> SNAMTQFEGFTNLYQVSKTLRFELIPQGKTLKHIQEQGFIEEDKARNDHYKELKPIIDRIYKTYADQCLQLVQLDWENLSAAIDSYRKEKTEETRNALIEEQATYRNAIHDYFIGRTDNLTDAINKRHAEIYKGLFKAELFNGKVLKQLGTVTTTEHENALLRSFDKFTTYFSGFYENRKNVFSAEDISTAIPHRIVQDNFPKFKENCHIFTRLITAVPSLREHFENVKKAIGIFVSTSIEEVFSFPFYNQLLTQTQIDLYNQLLGGISREAGTEKIKGLNEVLNLAIQKNDETAHIIASLPHRFIPLFKQILSDRNTLSFILEEFKSDEEVIQSFCKYKTLLRNENVLETAEALFNELNSIDLTHIFISHKKLETISSALCDHWDTLRNALYERRISELTGKITKSAKEKVQRSLKHEDINLQEIISAAGKELSEAFKQKTSEILSHAHAALDQPLPTTLKKQEEKEILKSQLDSLLGLYHLLDWFAVDESNEVDPEFSARLTGIKLEMEPSLSFYNKARNYATKKPYSVEKFKLNFQMPTLASGWDVNKEKCNGAILFVKNGLYYLGIMPKQKGRYKALSFEPTEKTSEGFDKMYYDYFPDAAKMIPKCSTQLKAVTAHFQTHTTPILLSNNFIEPLEITKEIYDLNNPEKEPKKFQTAYAKKTGDQKGYREALCKWIDFTRDFLSKYTKTTSIDLSSLRPSSQYKDLGEYYAELNPLLYHISFQRIAEKEIMDAVETGKLYLFQIYNKDFAKGHHGKPNLHTLYWTGLFSPENLAKTSIKLNGQAELFYRPKSRMKRMAHRLGEKMLNKKLKDQKTPIPDTLYQELYDYVNHRLSHDLSDEARALLPNVITKEVSHEIIKDRRFTSDKFFFHVPITLNYQAANSPSKFNQRVNAYLKEHPETPIIGIDRGERNLIYITVIDSTGKILEQRSLNTIQQFDYQKKLDNREKERVAARQAWSVVGTIKDLKQGYLSQVIHEIVDLMIHYQAVVVLENLNFGFKSKRTGIAEKAVYQQFEKMLIDKLNCLVLKDYPAEKVGGVLNPYQLTDQFTSFAKMGTQSGFLFYVPAPYTSKIDPLTGFVDPFVWKTIKNHESRKHFLEGFDFLHYDVKTGDFILHFKMNRNLSFQRGLPGFMPAWDIVFEKNETQFDAKGTPFIAGKRIVPVIENHRFTGRYRDLYPANELIALLEEKGIVFRDGSNILPKLLENDDSHAIDTMVALIRSVLQMRNSNAATGEDYINSPVRDLNGVCFDSRFQNPEWPMDADANGAYHIALKGQLLLNHLKESKDLKLQNGISNQDWLAYIQELRN

CRISPR-Cas12a uses guide RNAs to identify complementary ∼20-nucleotide sequences in genomic DNA to facilitate binding and double-strand cleavage. To engage DNA, Cas12a probes nucleotides immediately adjacent to 5′-TTTV-3′ protospacer adjacent motifs (PAMs) to test for guide RNA hybridization (1–3). We used cryo-electron microscopy (cryo-EM) to determine structures of a complex between Acidaminococcus sp. Cas12a-guide RNA and a PAM-containing non target DNA molecule. Using site-specific cross-linking to trap the otherwise transient encounter between the Cas12a ribonucleoprotein (RNP) and the DNA, we observed three classes of DNA conformations with different degrees of bending relative to a standard B-form helix.

We captured transient Cas12a RNP association with this substrate by introducing a disulfide crosslink between mutated amino acid N551C in Cas12a and an N4-cystamine-cyt(7) DNA modification. In all structures, the PAM sits in the Cas12a PAM-binding pocket. DNA in the candidate protospacer region is progressively bent and underwound from structures 1 to 3. In structure 1 and 3, key interactions between Lys548 and the PAM are absent. Adenosine in position (–2) on the target strand is 4.5–4.6 Å away from Lys548 side chain, placing it out of range for hydrogen bonding. In structure 1, there is no density for the loop 571–576 containing the Tyr575, and no side chain density for Lys613 precluding further interpretation of those regions. Gln656 interacts with the (+2) phosphate in structure 1, and with (+3) phosphate in structure 3 due to general PI domain shift towards the DNA and DNA bending, which brings (+3) phosphate closer to Gln656. The presence of full base-pairing without alternative base conformations in structures 1 and 2, where DNA distortion is less pronounced, suggests base flipping arises from protein-induced DNA bending. We propose that structures 1 through 3 represent progression through a conformational landscape of protein movement and concomitant DNA bending.> MGTFTLHQGQTNLIKSFFRNYYLNAELELPKDMELREFALQPFGSDTYVRHLSFSSSEELRDYLVNRNLPLHLFYSSARYQLPSARNMEEKAWMGSDLLFDIDADHLCKLRSIRFCPVCGNAVVSEKCERDNVETLEYVEMTSECIKRGLEQTRNLVEILEDDFGLKPKVYFSGNRGFHVQVDCYGNCALLDSDERKEIAEYVMGIGVPGYPGGSENAPGWVGRKNRGINGVTIDEQVTIDVKRLIRIPNSLHGKSGLIVKRVPNLDDFEFNETLSPFTGYTIFLPYI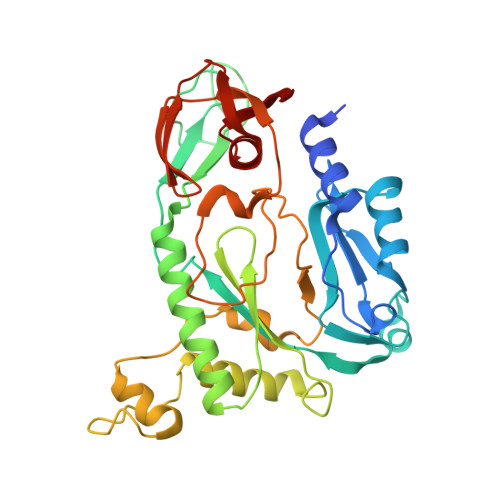TIETEVLGSIIKLNRGIPIKIKSSIGIYLHLRNLGEVKAYVR> GSDPLKIADQSVDLNLKLMKWRILPDLNLDIIKNTKVLLLGAGTLGCYVSRALIAWGVRKITFVDNGTVSYSNPVRQALYNFEDCGKPKAELAAASLK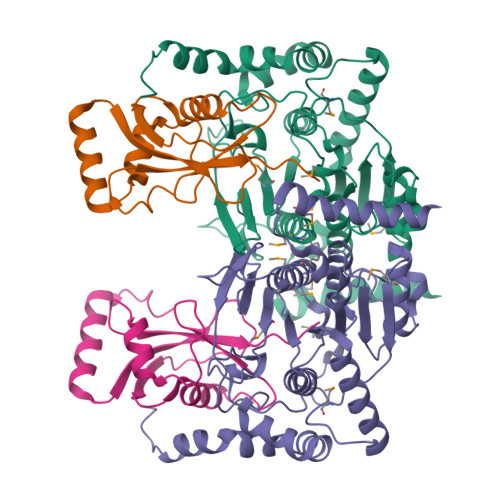RIFPLMDATGVKLSIPMIGHKLVNEEAQHKDFDRLRALIKEHDIIFLLVDSRESRWLPSLLSNIENKTVINAALGFDSYLVMRHGNRDEQSSKQLGCYFCHDVVAPTDSLTDRTLDQMSTVTRPGVAMMASSLAVELMTSLLQTKYSGSETTVLGDIPHQIRGFLHNFSILKLETPAYEHCPACSPKVIEAFTDLGWEFVKKALEHPLYLEEISGLSVIKQEVERLGNDVFEWEDDESDEIA;> GSMKSTFKSEYPFEKRKAESERIADRFKNRIPVICEKAEKSDIPEIDKRKYLVPADLTVGQFVYVIRKRIMLPPEKAIFIFVNDTLPPTAALMSAIYQEHKDKDGFLYVTYSGENTFG> MTFEEKLSKIYNEIANEISSMIPVEWEKVYTMAYIDDGGGEVFFNYTKPGSDDLNYYTNIPKEYNISVQVFDDLWMDLYDLFEELRDLFKEEDLEPWTSCEFDFTREGELKVSFDYIDWINSEFGQIGRQ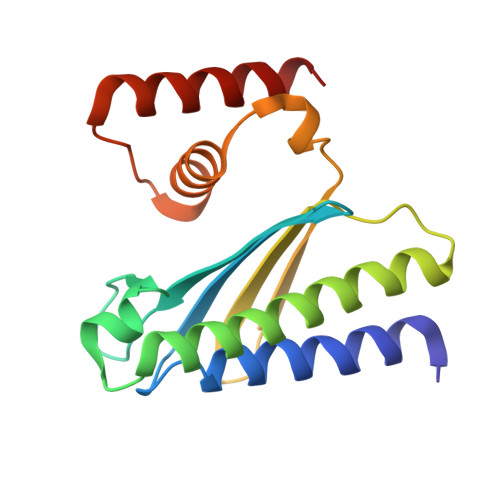NYYKYRKFGILPETEYEINKVKEIEQYIKELE>[4x]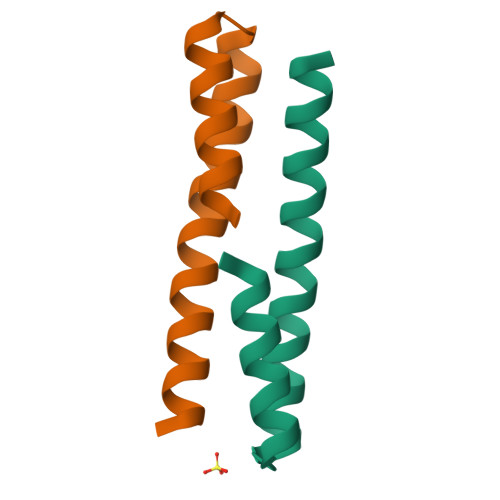XNLAALRSELQALRREGFSPERLAALESRLQALERRLAALRSRLQALRGX;>XCLAALRSELQALRREGFSPEELAALESELQALERELAALRSELQALRGX[4x]GABACULINE | C7 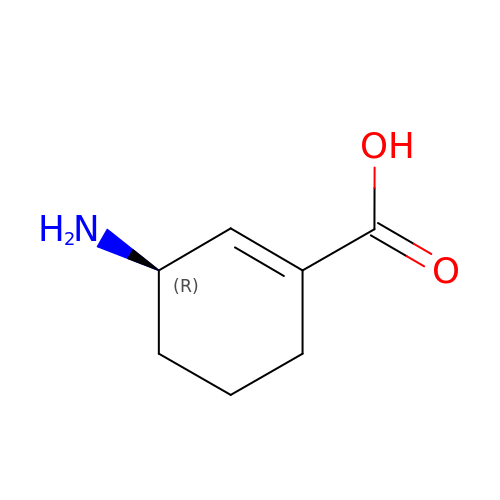H11 N O2 | ZCGFCFMGAXXBTD-ZCFIWIBFSA-N> GQGGKDMLSNGIKYLDVPYVAHTLEADGPEELVINCDEVDCTTLVEYVLAETLTPKLADGDISESAFADNLQKIRYRDGKIDGYTSRLHYIADWINNGVRNGFLQDVTGAMSPDTERLSISYMSSHPQLYKQLANSPENVAKMKKIEQSLSGKEVHYLPKAKLPADGLPWIKDGDIIAITTNTPGLDVAHMGIAFYAD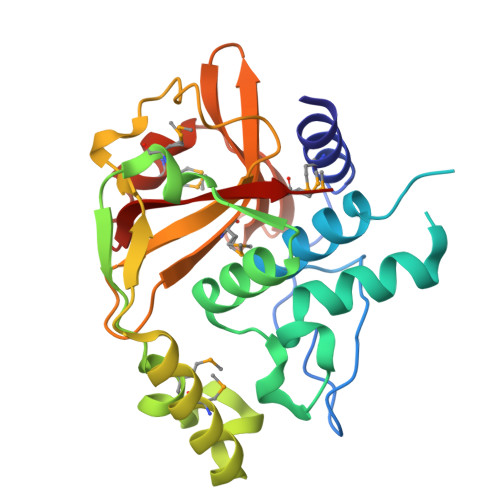NKLLLVHASSTDKKVVVSKVPLSQMLKDNNKWTGIRVLRMKK>MKNIHLIPYRVEQVTAAPPRIPEGVRMIQAPELWESAEHGKGNVVAVLDTGCQTDHPDLTARIAGGRNFTHDDGGDPERFEDYNGHGTHVAGTVAASLRDEEGVVGVAPLADLLVVKVLDKEGSGSYEGIIAGIHYAIDWRGPEGQKTTVISMSLGGPEDHPELYEAVKRAVDAGIPVICAAGNEGDDAHDTDEFAYPGAYGEVIQVGAVDFDRRIAPFSNTNNEIDLVAPGINIYSTYLEGKYASLSGTSMATPHVSGALALIRNISEREFDRELTEAELYAQLVRRTIPLGYPKTAEGNGLLALDILNKFEQLFKILSNSYANGLDRA[2x]

ISPs have key roles in cell cycle regulation, specifically in protein recycling by processing proteins during transition to the stationary phase. In the precursor protein, an N‐terminal pro‐peptide of typically 16‐20 residues binds across the active site and inhibits activity. ISPs are homodimeric, which contributes to making ISPs a structurally distinct family of subtilases.

ISPs are distinct from ESPs with regards to the N‐terminal pro‐peptide, their dimeric structure, and the sodium binding in the high affinity metal binding site, but details regarding their maturation are still unclear. To shed light on the latter, the crystal structure of the Asn3‐ISP was determined by X‐ray crystallography to a resolution of 1.3 Å. In addition to being the second unique structure of an ISP, it is the first structure of an ISP with a native catalytic triad, and it represents the highest resolution structure of this enzyme family to date. The structure of the ISP (residue 3‐310) is dimeric, with each monomer including an almost intact pro‐peptide bound across the active site. In the structure, there are 2 molecules of triethylene glycol (Peg3) symmetrically bound at the dimer interface distant from the active site, which may be adducts of Peg 1500 during crystallization or introduced during recombinant expression. The first 2 residues, 2 loop regions (residues 184‐191 and 217‐223), and the C‐terminal 20 residues are not defined in the electron density. Two distinct conformations were modelled in each monomer due to poor electron density: Monomer A, residues 248‐252 (including the catalytic triad residue Ser251) and Monomer B, residues 16‐20 (including parts of the pro‐peptide). In the crystals of Planococcus sp. AW02J18 ISP, calcium was not identified at any of the metal binding site. The 2 loop regions that are disordered (residues 184‐191 and 217‐223) in Planococcus sp. AW02J18 ISP are ordered in the structure that simulates the active state of the B. clausii ISP. The 2 residues form hydrophobic interactions to the side‐chain of Phe195 in our inactive structure and probably hinder this reorienting into the active conformation (this side‐chain appears to be shifted almost 15 Å in the active state). We thus conclude that the pro‐peptide, with the LIPY/F motif in a central position, is involved in inhibition.> YDSRWVKRLDRLRESKFYDPAPIIKEEEILEADKIHPLLKKVTPSWNSRRTGLLAYKIGMMSLWDGWGERHAVTVCQVDRCVVMDQRTLDKDGYEACVMGIGYKPIHKVTKPMLGVYIRSQIEPKSRIAEFKCSSDCLLPVGHEMSVRHFTPGQQVFVSGWSKDKGYLGVKKRWGFAGQ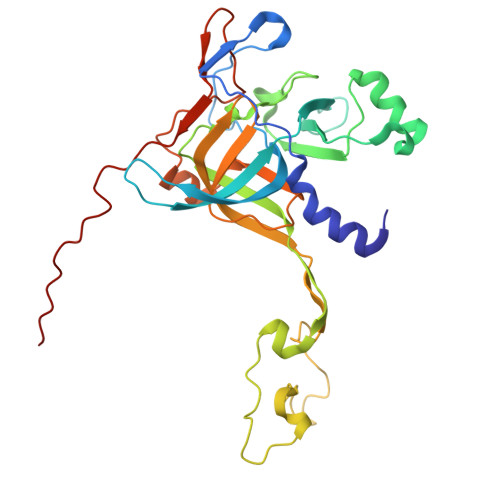NASHGVEAKAHSSPGSIGQSKTVNVVWRFKKMAGHAGGDPRVVNCKVFRIEAQRNLIFLKGCVPGYKGSLIKISDARGKTHHRHNRHIPLHFPTFVPEPGVSYPVTLECPDAEQDPFLYPEIAIADK>SQCSGIDKRDFIQGVSGGTWVDVVLDRKGCVTISATGKPTIDVRMVKMEASNLASVRTYCLEASTSEISSVNGCPSTTEAHNDKRKDSTYLCERSYPDRGWGNGCGLFGRGSLDTCVKFACSKKMAGHAISRENIVITAAVSVHGHSGAESDDRSQRKSRKELAELTITFKSSIVEADLGDYGKVQFECLMDFGIDLDDVYTADMSGKWWLVKRDWYHDIALPWTAPSADFWHDMDRLVEFSTPHATKQSVYTLGDQEGAMSTALGDAAVIEYMSSGSKVVFRTGFLKCRVKMENLRLKGSTYMQCSKEFSILKRPTATPYGTVIMQVKYAQTDVPCRVPVGVHERPGGEQVGRIITAHPIILQQNDALVIEVEPPFGDSVIEIGLGTTKIVEQWHRDGSSIGAAFTSTMKGVERMALLGEHAWDFGSVGGFFNSMGKAIHSVFGGLFRAVFGGMSWISKVLIGAILMWLGVSAREKTLAMSLITVGAILLYLSTMTNAVS[3x];>[3x]SIMIPTH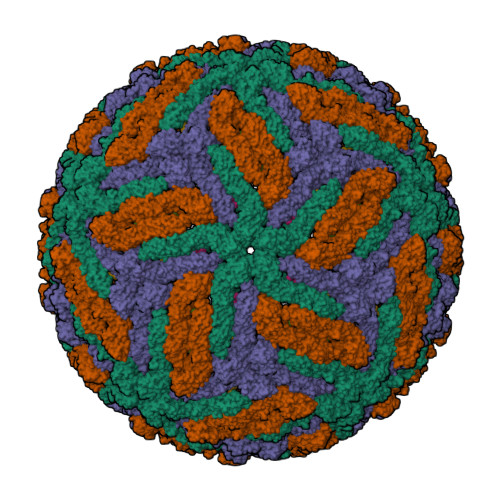STGGLHQGTEGWHRTNNVKNFLMRVEKWSLRNPGYTALIAILGWTLGTTTAQKVIFIALLLMIAPVYG>MATPSMMPQWSYMHISGQDASEYLSPGLVQFARATETYFSLNNKFRNPTVAPTHDVTTDRSQRLTLRFIPVDREDTAYSYKARFTLAVGDNRVLDMASTYFDIRGVLDRGPTFKPYSGTAYNALAPKGAPNPCEWDEAATALEINLEEEDDDNEDEVDEQAEQQKTHVFGQAPYSGINITKEGIQIGVEGQTPKYADKTFQPEPQIGESQWYETEINHAAGRVLKKTTPMKPCYGSYAKPTNENGGQGILVKQQNGKLESQVEMQFFSTTEATAGNGDNLTPKVVLYSEDVDIETPDTHISYMPTIKEGNSRELMGQQSMPNRPNYIAFRDNFIGLMYYNSTGNMGVLAGQASQLNAVVDLQDRNTELSYQLLLDSIGDRTRYFSMWNQAVDSYDPDVRIIENHGTEDELPNYCFPLGGVINTETLTKVKPKTGQENGWEKDATEFSDKNEIRVGNNFAMEINLNANLWRNFLYSNIALYLPDKLKYSPSNVKISDNPNTYDYMNKRVVAPGLVDCYINLGARWSLDYMDNVNPFNHHRNAGLRYRSMLLGNGRYVPFHIQVPQKFFAIKNLLLLPGSYTYEWNFRKDVNMVLQSSLGNDLRVDGASIKFDSICLYATFFPMAHNTASTLEAMLRNDTNDQSFNDYLSAANMLYPIPANATNVPISIPSRNWAAFRGWAFTRLKTKETPSLGSGYDPYYTYSGSIPYLDGTFYLNHTFKKVAITFDSSVSWPGNDRLLTPNEFEIKRSVDGEGYNVAQCNMTKDWFLVQMLANYNIGYQGFYIPESYKDRMYSFFRNFQPMSRQVVDDTKYKDYQQVGILHQHNNSGFVGYLAPTMREGQAYPANFPYPLIGKTAVDSITQKKFLCDRTLWRIPFSSNFMSMGALTDLGQNLLYANSAHALDMTFEVDPMDEPTLLYVLFEVFDVVRVHRPHRGVIETVYLRTPFSAGNATT[12x];> MRRAAMYEEGPPPSYESVVSAAPVAAALGSPFDAPLDPPFVPPRYLRPTGGRNSIRYSELAPLFDTTRVYLVDNKSTDVASLNYQNDHSNFLTTVIQNNDYSPGEASTQTINLDDRSHWGGDLKTILHTNMPNVNEFMFTNKFKARVMVSRLPTKDNQVELKYEWVEFTLPEGNYSETMTIDLMNNAIVEHYLKVGRQNGVLESDIGVKFDTRNFRLGFDPVTGLVMPGVYTNEAFHPDIILLPGCGVDFTHSRLSNLLGIRKRQPFQEGFRITYDDLEGGNIPALLDVDAYQASLKDDTEQGGGGAGGSNSSGSGAEENSNAAAAAMQPVEDMNDHAIRGDTFATRAEEKRAEAEAAAEAAAPAAQPEVEKPQKKPVIKPLTEDSKKRSYNLISNDSTFTQYRSWYLAYNYGDPQTGIRSWTLLCTPDVTCGSEQVYWSLPDMMQDPVTFRSTRQISNFPVVGAELLPVHSKSFYNDQAVYSQLIRQFTSLTHVFNRFPENQILARPPAPTITTVSENVPALTDHGTLPLRNSIGGVQRVTITDARRRTCPYVYKALGIVSPRVLSSRTF;> MMQDATDPAVRAALQSQPSGLNSTDDWRQVMDRIMSLTARNPDAFRQQPQANRLSAILEAVVPARANPTHEKVLAIVNALAENRAIRPDEAGLVYDALLQRVARYNSGNVQTNLDRLVGDVREAVAQRERAQQQGNLGSMVALNAFLSTQPANVPRGQEDYTNFVSALRLMVTETPQSEVYQSGPDYFFQTSRQGLQTVNLSQAFKNLQGLWGVRAPTGDRATVSSLLTPNSRLLLLLIAPFTDSGSVSRDTYLGHLLTLYREAIGQAHVDEHTFQEITSVSRALGQEDTGSLEATLNYLLTNRRQKIPSLHSLNSEEERILRYVQQSVSLNLMRDGVTPSVALDMTARNMEPGMYASNRPFINRLMDYLHRAAAVNPEYFTNAILNPHWLPPPGFYTGGFEVPEGNDGFLWDDIDDSVFSPQPQTLLELQQREQAEAALRKESFRRPSSLSDLGAAAPRSDASSPFPSLIGSLTSTRTTRPRLLGEEEYLNNSLLQPQREKNLPPAFPNNGIESLVDKMSRWKTYAQEHRDVPGPRPPTRRQRHDRQRGLVWEDDDSADDSSVLDLGGSGNPFAHLRPRLGRMF;>M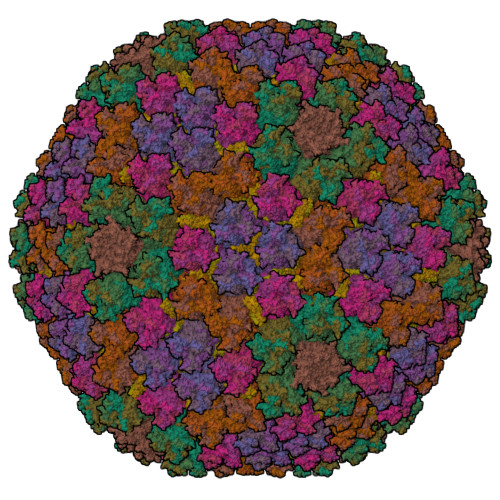SKEIPTPYMWSYQPQMGLAAGAAQDYSTRINYMSAGPHMISRVNGIRAHRNRILLEQAAITTTPRNNLNPRSWPAALVYQESPAPTTVVLPRDAQAEVQMTNSGAQLAGGFRHRVRSPGQGITHLTIRGRGIQLNDESVSSSLGLRPDGTFQIGGAGRPSFTPRQAILTLQTSSSEPRSGGIGTLQFIEEFVPSVYFNPFSGPPGHYPDQFIPNFDAVKDSADGYD[2x];>[4x]MSTNSFDGSIVSSYLTTRMPPWAGVRQNVMGSSIDGRPVLPANSTTLTYETVSGTPLETAASAAASAAAATARGIVTDFAFLSPLASSAASRSSARDDKLTALLAQLDSLTRELNVVSQQLLDLRQQVSALKASSPPNAV;>[3x]MEDINFASLAPRHGSRPFMGNWQDIGTSNMSGG;> GLRFPSKMFGG;> AFSWGSLWSGIKNFGSTVKNYGSKAWNSSTGQMLRDKLKEQNFQQKVVDGLASGISGVVDLANQAVQNKINSKLDPRPPVEEPPPAVETVSPEGRGEKRPRPDREETLVTQIDEPPSYEEALKQGLPTTRPIAPMATGVLGQHTPVTLDLPPPADTQQKPVLPGPTAVVVTRPSRASLRRAASGPRSLRPVASGNWQSTLNSIVGLGVQSLKRRRCF> GSHMRFDEFGNIITDSAVAEEPEPELPGVTEEALRLKEAALEELAAQEVTAPLVPLAVSAFLTSRKKAAAAELADWMQSPEGQASSLESIGRSLSRRNHGRSRAVVLAHDHDEAIKGLRAVAAGKQAPNVFSVDGPVTTGPVWVLAGFGAQHRKMGKSLYLRNEVFAAWIEKVDALVQDELGYSVLELILDDAQDYGIETTQVTIFAIQIALGELLRHHGAKPAAVIGQSLGEAASAYFAGGLSLRDATRAICSRSHLMGEGEAMLFGEYIRLMALVEYSADEIREVFSDFPDLEVCVYAAPTQTVIGGPPEQVDAILARAEAEGKFARKFATKGASHTSQMDPLLGELTAELQGIKPTSPTCGIFSTVHEGRYIKPGGEPIHDVEYWKKGLRHSVYFTHGIRNA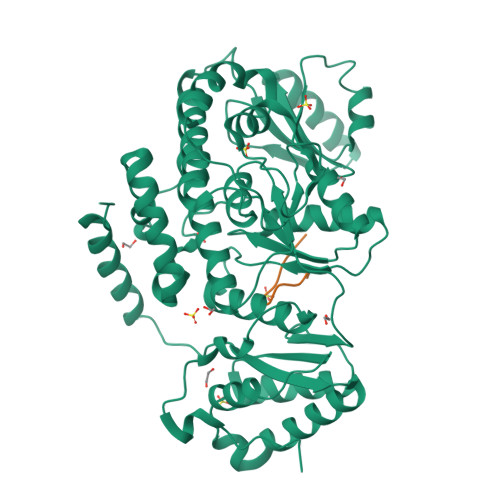VDSGHTTFLELAPNPVALMQVALTTADAGLHDAQLIPTLARKQDEVSSMVSTMAQLYVYGHDLDIRTLFSRASGPQDYANIPPTRF;> SDKENFWGMAVA> SNARKIKTEPKQMHEDYCFQCGDGGELVMCDKKDCPKAYHLLCLNLTQP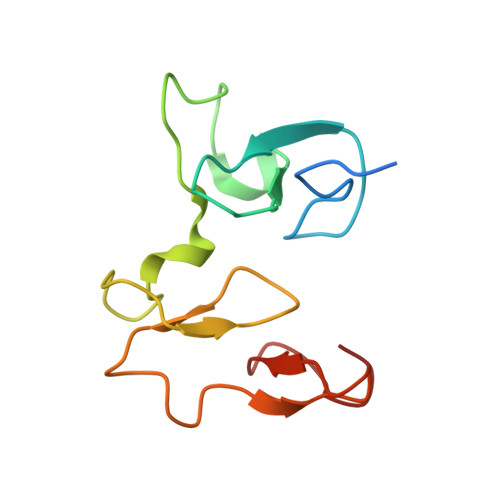PYGKWECPWHQCDECSSAAVSFCEFCPHSFCKDHEKGALVPSALEGRLCCSEHDPMAP> MNYTKFDVKNWVRREHFEFYRHRLPCGFSLTSKIDITTLKKSLDDSAYKFYPVMIYLIAQAVNQFDELRMAIKDDELIVWDSVDPQFTVFHQETETFSALSCPYSSDID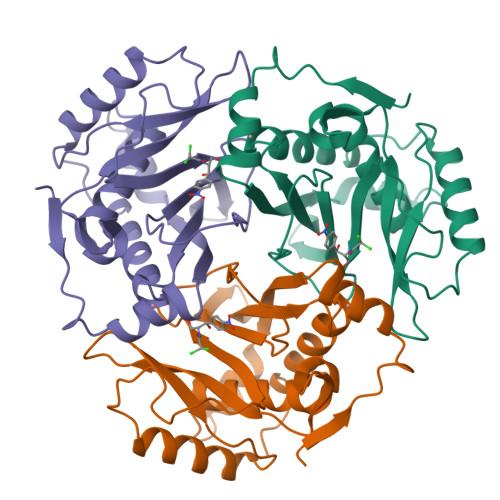QFMVNYLSVMERYKSDTKLFPQGVTPENHLNIAALPWVNFDSFNLNVANFTDYFAPIITMAKYQQEGDRLLLPLSVQVHHAVCDGFHVARFINRLQELCNSKLK3-CHLORO-9-ETHYL-6,7,8,9,10,11-HEXAHYDRO-7,11-METHANOCYCLOOCTA[B]QUINOLIN-12-AMINE | C18 H19 Cl N2 | 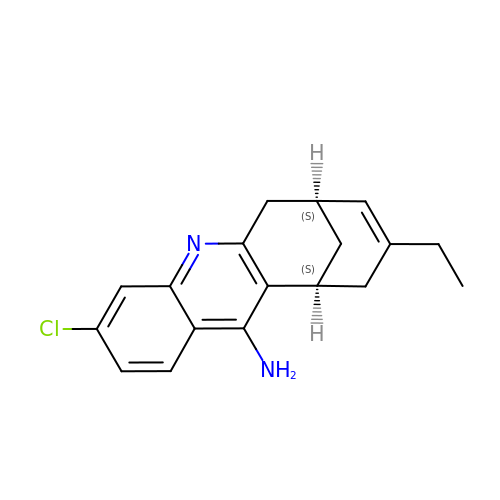QTPHSDHUHXUYFE-NWDGAFQWSA-N oligomycin B | C45 H72 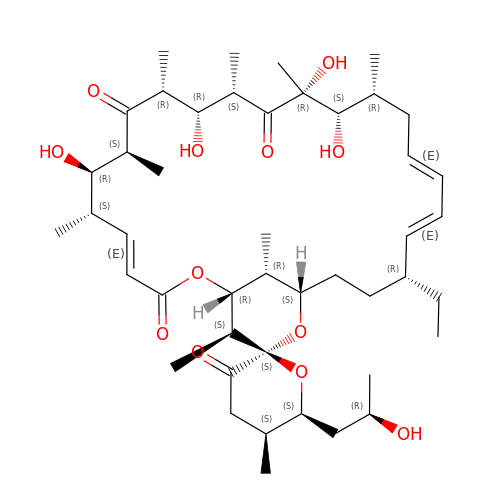O12 | QPRQJOHKNJIMGN-WVUAJZTGSA-N1-[4-[2-(4-methoxyphenyl)-5-methyl-pyrrolo[2,3-b]pyrazin-6-yl]piperidin-1-yl]ethanone 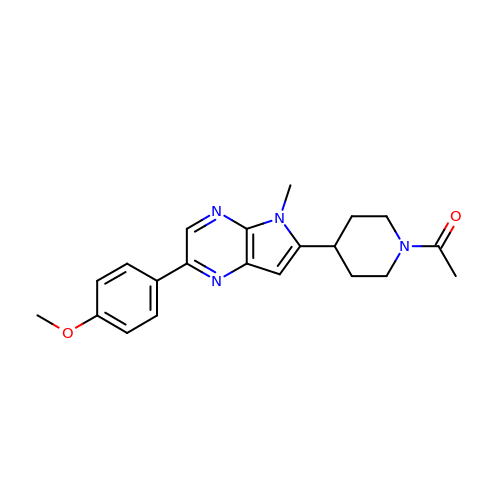| C21 H24 N4 O2 | HEAGFUMRBLFGAD-UHFFFAOYSA-N>[5x]GSHMGGVEVLNIITGPDSTTEIELYLEPRMGINSPTGDKKEWYGYSEVIHHADGYDNNLLSIQMPQYSCARVQLPMLNTDMTSDTLMMWEAVSCKTEIVGIGSLISVHLLEAKMA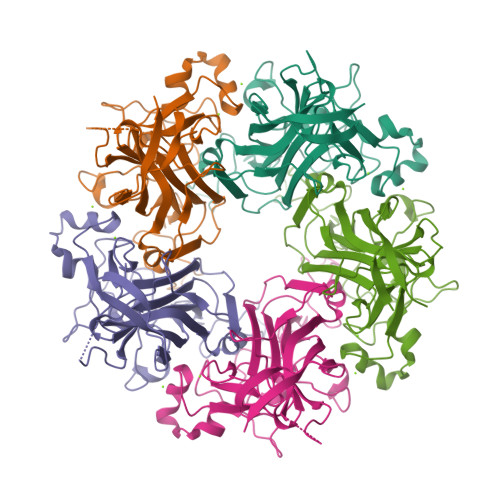AKEGGDGPSQPIEGMNYHMFAVGGEPLDLQGIESNALTKYASAIPPKTIHPNDIAKLAEEEKPQLQGLVPKAKARLDKDGFYPIEEWSPDPSRNENSRYFGSFVGGLNTPPNLQFTNAVTTVLLDENGVGPLCKGDGLFVSAADICGVMVKADNEAIRYRGLPRYFKVTLRKRAVKN>CUGGGCGG[2x];>CCGC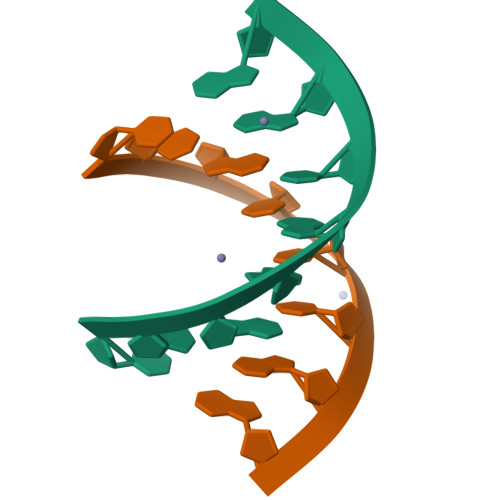CUGG[2x]> SLSNKLTLDKLDVKGKRVVMRVDFNVPMKNNQITNNQRIKAAVPSIKFCLDNGAKSVVLMSHLGRPDGVPMPDKYSLEPVAVELKSLLGKDVLFLKDCVGPEVEKACANPAA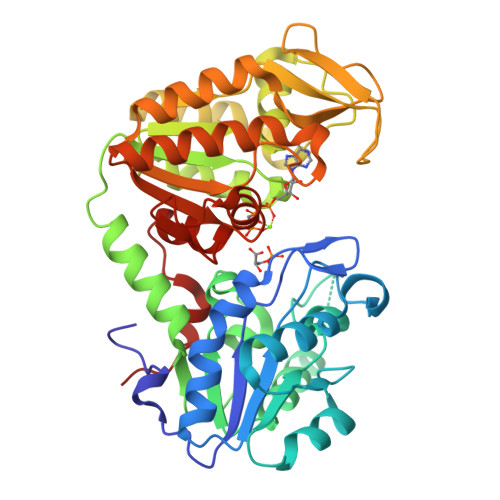GSVILLENLRFHVEEEGKGKDASGNKVKAEPAKIEAFRASLSKLGDVYVNDAFGTAHRAHSSMVGVNLPQKAGGFLMKKELNYFAKALESPERPFLAILGGAKVADAIQLINNMLDKVNEMIIGGGMAFTFLKVLNNMEIGTSLFDEEGAKIVKDLMSKAEKNGVKITLPVDFVTADKFDENAKTGQATVASGIPAGWMGLDCGPESSKKYAEAVTRAKQIVWNGPVGVFEWEAFARGTKALMDEVVKATSRGCITIIGGGDTATCCAKWNTEDKVSHVSTGGGASLELLEGKVLPGVDALSNI(2R)-2-(alpha-D-glucopyranosyloxy)-3-hydroxypropanoic acid | C9 H16 O9 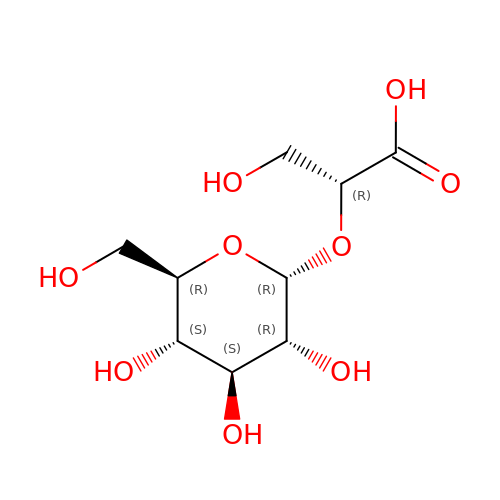| DDXCFDOPXBPUJC-CECBSOHTSA-N N-[2-(6-AMINO-4-METHYLPYRIDIN-2-YL)ETHYL]-4-CYANOBENZAMIDE 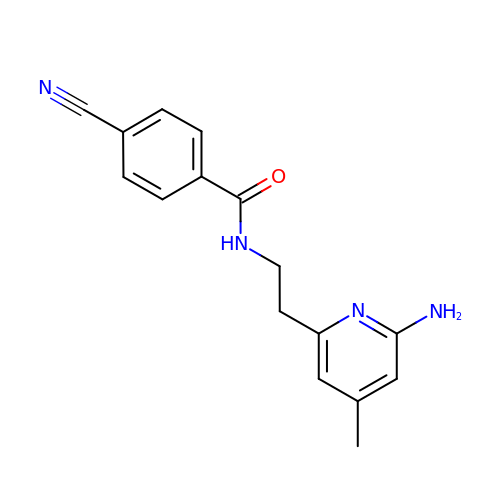| C16 H16 N4 O | QINCZVSBLITNRD-UHFFFAOYSA-N>MVPISPIETVPVKLKPGMDGPKVKQWPLTEEKIKALVEICTEMEKEGKISKIGPENPYNTPVFAIKKKDSTKWRKLVDFRELNKRTQDFWEVQLGIPHPAGLKQKKSVTVLDVSAAFYSVPLDKDFRKYTAFTIPSINNETPGIRYQYNVLPMGWKGSPALLQSSMTKILEPFRKQNPDIVIYQYMDDLYVGSDLEIGQHRTKIEELRQHLLRWGFTTPDKKHQKEPPFLWMGYELHPDKWTVQPIVLPEKDSWTVNDIQKLVGKLNWASQIYAGIKVRQLSKLLRGTKALTEVVPLTEEAELELAENREILKEPVHGVYYDPSKDLIAEIQKQGQGQWTYQIYQEPFKNLKTGKYARMKGAHTNDVKQLTEAVQKIATESIVIWGKTPKFKLPIQKETWEAWWTEYWQATWIPEWEFVNTPPLVKLWYQLEKEPIIGAETFYVDGAANRETKLGKAGYVTDRGRQKVVPLTDTTNQKTELQAIHLALQDSGLEVNIVTDSQYALGIIQAQPDKSESELVSQIIEQLIKKEKVYLAWVPAHKGIGGNEQVDKLVSAG[2x];>[2x]MAHHHHHHALEVLFQGPISPIETVPVKLKPGMDGPKVKQWPLTEEKIKALVEICTEMEKEGKISKIGPENPYNTPVFAIKKKDSTKWRKLVDFRELNKRTQDFWEVQLGIPHPAGLKQKKSVTVLDVGDAYFSVPLDKDFRKYTAFTIPSINNETPGIRYQYNVLPQGWKGSPAIFQSSMTKILEPFRKQNPDIVIYQYMDDLYVGSDLEIGQHRTKIEELRQHLLRWGFTTPDKKHQKEPPFLWMGYELHPDKWTVQPIVLPEKDSWTVNDIQKLVGKLNWASQIYAGIKVRQLSKLLRGTKAL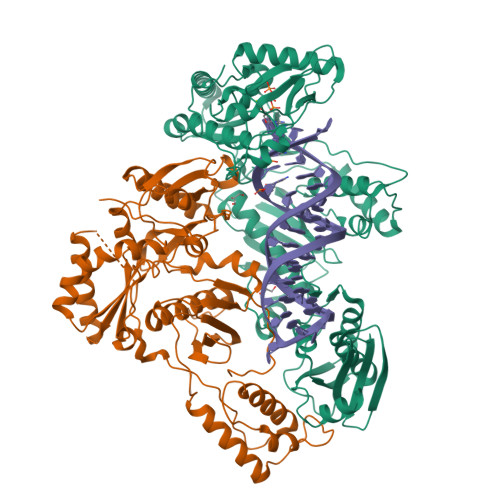TEVVPLTEEAELELAENREILKEPVHGVYYDPSKDLIAEIQKQGQGQWTYQIYQEPFKNLKTGKYARMKGAHTNDVKQLTEAVQKIATESIVIWGKTPKFKLPIQKETWEAWWTEYWQATWIPEWEFVNTPPLVKLWYQ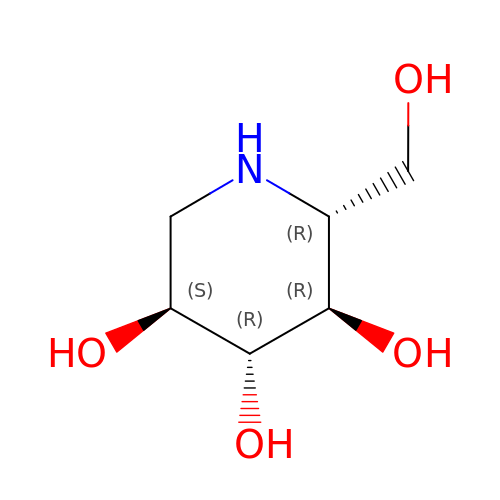1-DEOXYNOJIRIMYCIN | C6 H13 N O4 | LXBIFEVIBLOUGU-JGWLITMVSA-N>MKTIIINGVQFNTDEDTTILKFARDNNIDISALCFLNNCNNDINKCEICTVEVEGTGLVTACDTLIEDGMIINTNSDAVNEKIKSRISQLLDIHEFKCGPCNRRENCEFLKLVIKYKARASKPFLPKDKTEYVDERSKSLTVDRTKCLLCGRCVNACGKNTETYAMKFLNKNGKTIIGAEDEKCFDDTNCLLCGQCIIACPVAALSEKSHMDRVKNALNAPEKHVIVAMAPSVRASIGELFNMGFGVDVTGKIYTALRQLGFDKIFDINFGADMTIMEEATQLVQRIENNGPFPMFTSCCPGWVRQAENYYPELLNNLSSAKSPQQIFGTASKTYYPSISGLDPKNVFTVTVMPCTSKKFEADRPQMEKDGLRDIDAVITTRELAKMIKDAKIPFAKLEDSEADPAMGEYSGAGAIFGATGGVMEAALRSAKDFAENAELEDIEYKQVRGLNGIKEAEVEINNNKYNVAVINGASNLFKFMKSGMINEKQYHFIEVMACHGGCVNGGGQPHVNPKDLEKVDIKKVRASVLYNQDEHLSKRKSHENTALVKMYQNYFGKPGEGRAHEILHFKYKKSAWSHPQFEK[2x]

[FeFe]-hydrogenases represent one of natures’ most effective classes of redox enzymes catalyzing the reversible reduction of protons to dihydrogen (H2) at turnover frequencies of up to 9000 s-11–3. With their low catalytic over-potential, [FeFe]-hydrogenases represent excellent models for a regenerative and likewise economically feasible H2 production. Their active center (“H-cluster”) can be structured into a standard [4Fe-4S]-cluster ([4Fe]H) and a diiron site ([2Fe]H). Theoretical studies suggest that the most probable PT pathway comprises of strictly conserved residues E282, S319, E279, and C299 (from surface to H-cluster, numbering corresponds to CpI), including two protein-bound water molecules (Wat826, Wat1120 4XDC19, chain B) located between E279 and C29915,16,20. In this study, site-directed mutagenesis (SDM) is used to investigate the PT pathway of two [FeFe]-hydrogenases, namely CpI and HydA1, which represent the largest (M3) and smallest (M1) type of monomeric [FeFe]-hydrogenases, respectively.

Corresponding to earlier crystal structure data, for all CpI variants a space group of P1 21 1 was observed with two copies in the asymmetric unit cell (chain A and B). In variant E282QCpI, the glutamine residue is potentially stabilized by two hydrogen bonds  (H-bonds) unrelated to the putative PT pathway thus, blocking PT and rendering the enzyme largely inactive. Additionally, the two different conformations of Q282CpI in chain A and B indicate structural flexibility at the entrance of the PT pathway, which may support the residual activity measured for this variant. Corresponding substitutions in CpI and HydA1 had similar effects on H2-release activity, except for variants E282QCpI (8.2%) and E144QHydA1 (0.4%). In case of E282CpI, a substitution for aspartic acid shifted the optimum only slightly to pH 7.5 while an exchange to alanine or glutamine rendered the enzyme most active at pH 7 and 6, respectively.>SPATLPQLTPTLVSLLEVIEPEVLYAGYDGTVPDTTWRIMTTLNMLGGRQVIAAVKWAKAIPGFRNLHLDDQMTLLQYSWMSLMAFALGWRSYRQSSGNVLCFAPDLIINEQRMGLPYMYDQCKQMLFVSSELKRLQVSYEEYLCMKTLLLFSSVPKEGLKSQELFDEIRMTYIKELGKAIVKREGNSSQNWQRFYQLTKLLDSMHE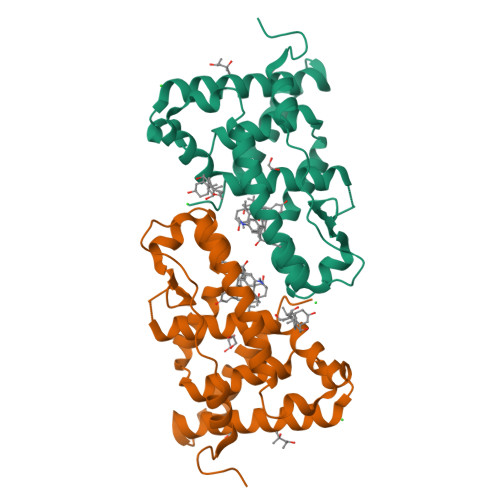NVTWLKPESTSHFSL[2x]> NGIAAMLQRH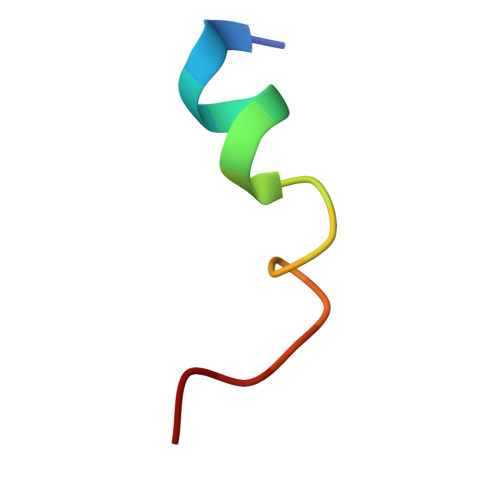SRKRFQL> LQTET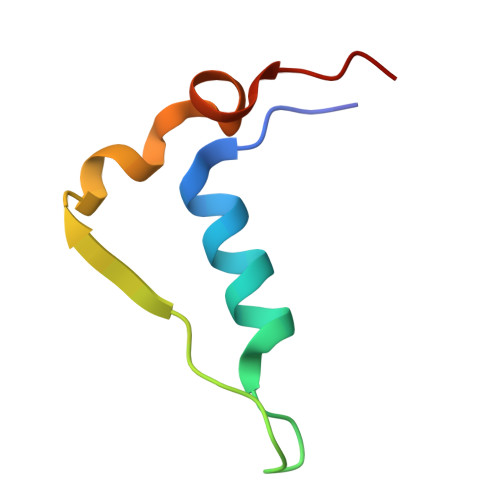LHQQYELVKRRTAPVGYSYGSHVMQYGDVGISKDNLDLYMGTNPAN8-butyl-1-methyl-7-(5-methyl-1H-indazol-4-yl)-1H-imidazo[2,1-f]purine-2,4(3H,8H)-dione 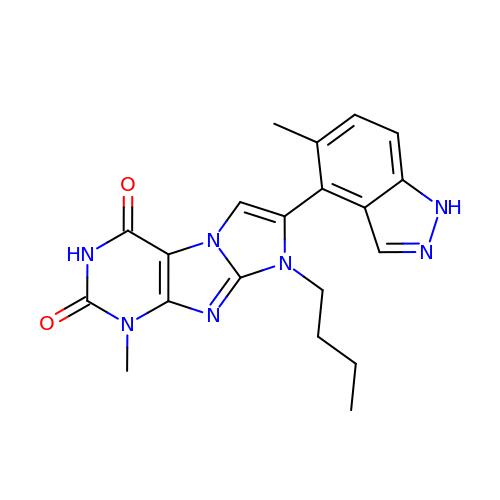| C20 H21 N7 O2 | DQROUBDXZUEWBE-UHFFFAOYSA-N> MREYKLVVLGSGGVGKSALTVQFVQGIFVDEYDPTIEDSYRKQVEVDCQQCMLEILDTAGTEQFTAMRDLYMKNGQGFALVYSITAQSTFNDLQDLREQILRVKDTEDVPMILVGNKCDLEDERVVGKEQGQNLARQWCNCAFLESSAKSKINVNEIFYDLVRQINR;> PSKT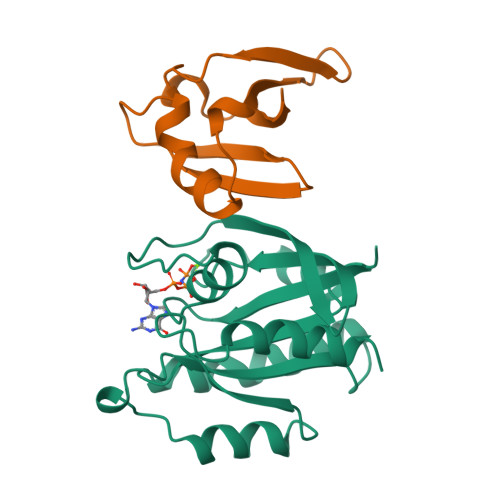SNTIRVFLPNKQRTVVNVRNGMSLHDCLMKALKVRGLQPECCAVFRLLHEHKGKKARLDWNTDAASLIGEELQVDFL>[4x]PAKKPYNKIVSHLLVAEPEKIYAMPDPTVPDSDIKALTTLCDLADRELVVIIGWAKHIPGFSTLSLADQMSLLQS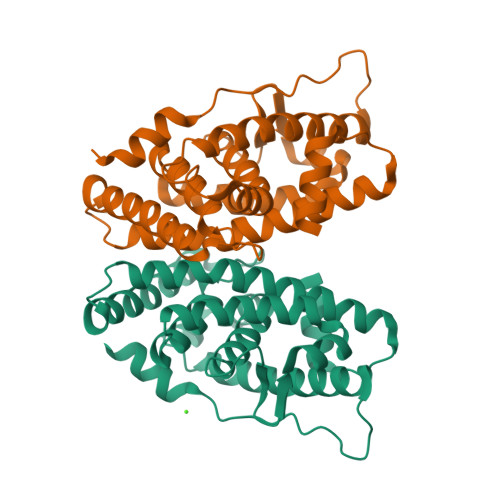AWMEILILGVVYRSLSFEDELVYADDYIMDEDQSKLAGLLDLNNAILQLVKKYKSMKLEKEEFVTLKAIALANSDSMHIEDVEAVQKLQDVLHEALQDYEAGQHMEDPRRAGKMLMTLPLLRQTSTKAVQHFYNIKLEGKVPMHKLFLEMLEAKV> MSSSGTPDLPVLLTDLKIQYTKIFINNEWHDSVSGKKFPVFNPATEEELCQVEEGDKEDVDKAVKAARQAFQIGSPWRTMDASERGRLLYKLADLIERDRLLLATMESMNGGKLYSNAYLSDLAGCIKTLRYCAGWADKIQGRTIPIDGNFFTYTRHEPIGVCGQIIPWNFPLVMLIWKIGPALSCGNTVVVKPAEQTPLTALHVASLIKEAGFPPGVVNIVPGYGPTAGAAISSHMDIDKVAFTGSTEVGKLIKEAAGKSNLKRVTLELGGKSPCIVLADADLDNAVEFAHHGVFYHQGQCCIAASRIFVEESIYDEFVRRSVERAKKYILGNPLT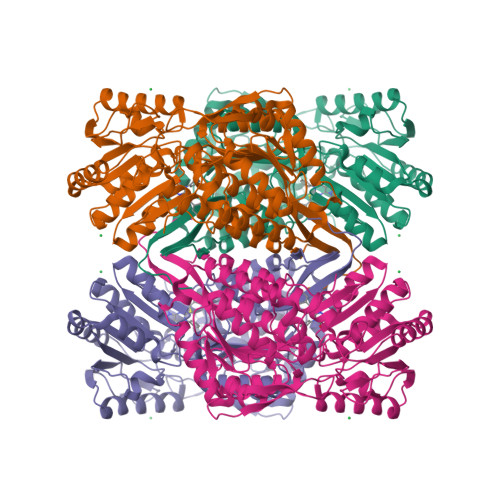PGVTQGPQIDKEQYDKILDLIESGKKEGAKLECGGGPWGNKGYFVQPTVFSNVTDEMRIAKEEIFGPVQQIMKFKSLDDVIKRANNTFYGLSAGVFTKDIDKAITISSALQAGTVWVNCYGVVSAQCPFGGFKMSGNGRELGEYGFHEYTEVKTVTVKISQKNS> VVGGTDADEGEWPWQVSLHALGQGHICGASLISPNWLVSAAHCYIDDRGFRYSDPTQWTAFLGLHDQSQRSAPGVQERRLKRIIS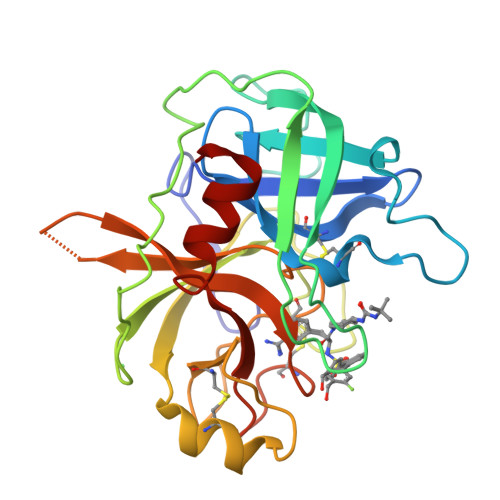HPFFNDFTFDYDIALLELEKPAEYSSMVRPISLPDASHVFPAGKAIWVTGWGHTQYGGTGALILQKGEIRVINQTTCENLLPQQITPRMMCVGFLSGGVDSCQGDSGGPLSSVEADGRIFQAGVVSWGDGCAQRNKPGVYTRLPLFRDWIKENTGV> MGHHHHHHHHHHSSGHIEGRHMGDEKCGKSLKLGNISNQTNQETITQSLS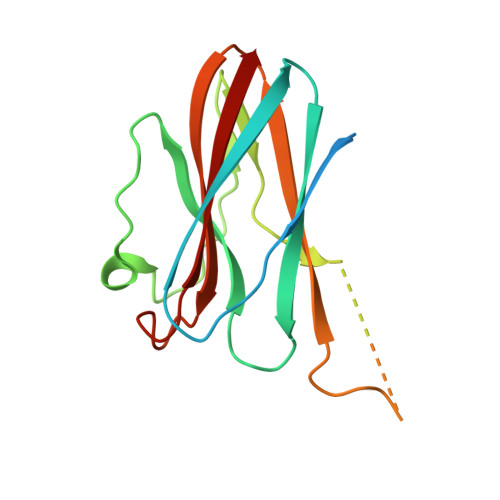VGEILCIDLEGNAGTGYLWVLLGIHKDEPIINPENFPTKLTKKSFFSEEISVTQPKKYKIDEHDSSKNVNREIESPEQKESDSKPKKPQMQLLGGPDRMRSVIKGHKPGKYYIVYSYYRPFSPTSGANTKIIYVTVQ(2R)-N-[(2R)-2-(DIHYDROXYBORYL)-1-L-PROLYLPYRROLIDIN-2-YL]-N-[(5R)-5-(DIHYDROXYBORYL)-1-L-PROLYLPYRROLIDIN-2-YL]-L-PROLINAMIDE 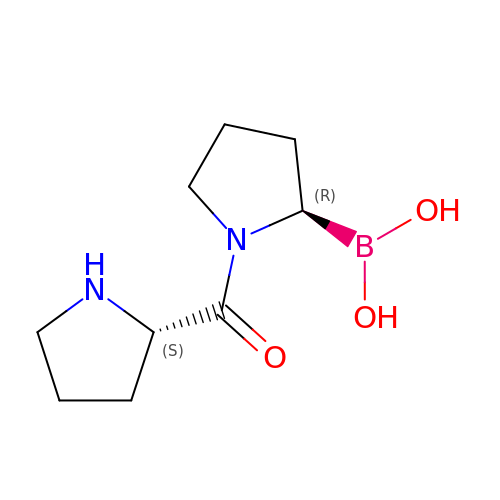| C9 H17 B N2 O3 | XSBZZZGVAIXJLD-YUMQZZPRSA-N> DEGCLPDWSSYKGHCYKVFKVEKTWADAEKFCKELVNGGHLMSVNS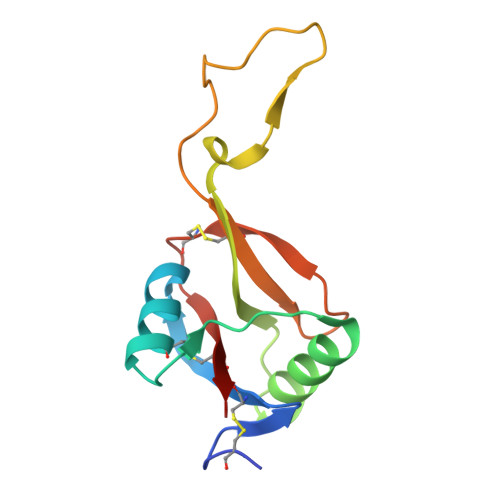REEGEFISKLALEKMRIVLVWIGLSHFWRICPLRWTDGARLDYRALSDEPICFVAESFHNKWIQWTCNRKKSFVCKYRV In this paper we describe a novel filamentous double-stranded (ds) DNA virus that infects a host living in nearly boiling acid, and show how components of the virion (proteins and lipids) can diverge considerably while preserving the overall virion organization and mode of the dsDNA packaging. Like most archaeal filamentous viruses, SFV1 contains an envelope. The results revealed that the two most prominent bands contained proteins VP4 and VP5, with apparent molecular masses of about 16 and 23 kDa, which are encoded by ORF23 and ORF24, respectively. Surprisingly, VP4 and VP5 assemble to form a pseudo-symmetric heterodimer, which wraps around the DNA, in a manner similar to the symmetrical capsid homodimer in SIRV2 and the pseudo-symmetrical heterodimer in AFV1.

By trial-and-error, the correct symmetry (which was 17.14 units/turn) revealed a largely α-helical protein capsid, while incorrect symmetry values gave rise to density that was uninterpretable. The three-dimensional reconstruction showed a total diameter of ~270 Å, and that the nucleocapsid within the outer membrane had a helical pitch of ~47 Å. The asymmetric unit was shown to contain VP4, VP5 and 12 bp of DNA, since the 3.7 Å resolution of the reconstruction allowed building an unambiguous atomic model for both VP4 and VP5 as well as for the DNA. The DNA exists in the A-form, as has been shown for SIRV28 and AFV19. Since there are 12 bp per asymmetric unit, with 17.14 units/turn, there are ~120 asymmetric units in seven 47 Å pitch helical turns. This means that there are 1440 bp in 127 turns (120 local right-handed turns and seven right-handed superhelical turns), so the DNA has a twist of 11.3 bp/turn. An interesting difference between SFV1 and both SIRV2 and AFV1 is that the protein subunits contain N-terminal portions that project into the DNA groove. In VP5 approximately six or seven residues can be seen making a deep insertion into the hollow core of the DNA (in A-DNA there is such a hollow core, which does not exist in B-DNA). In VP4 no density exists for the first three residues, but two or three residues at the N-terminus can be seen partially inserting into the DNA. In contrast to the compact dimers in SIRV2 and AFV1, VP5 contains a small C-terminal domain containing two short helices that projects away from the dimer. This small VP5 domain makes extensive contacts with a VP4 subunit in an adjacent helical turn as well as with the C-terminal domain from two other VP5 subunits in the same helical turn.

>[26x]MARKRTSKNDPLRMYLNYVRKLQTMGDAYDESAKYRIANFENGFKSLHMVENEFKQYLANVIDEAIKSGASPQDLPYVNEIKLALMKIFTSWLKYSNEKLGANEIAINVAGTATMTLTENLYGTRVSCEEAVSLINSIFAVWVGVEPFEAEEREGACLVTPRSPLPPVPISSPTGFSAPIQEVLQAKSPEEIIGVKGGA;>MPSRRTGITTEDAITKYSVKAKTEQTAYKNATKDMVVQAQNIMNFYSVVNQALIPWLNAHGVGGNLRILYRQLANEYVKVLNTKQSGEVIKRLKIALRHKYWLRGLDEAMLDEFMDYIDSLKSTTTNYIIFNMQSSK[26x]>[2x]GSGGSGKVVKFSYMWTINNFSFCREEMGEVIKSSTFSSGANDKLKWCLRVNPKGLDEESKDYLSLYLLLVSCPKSEVRAK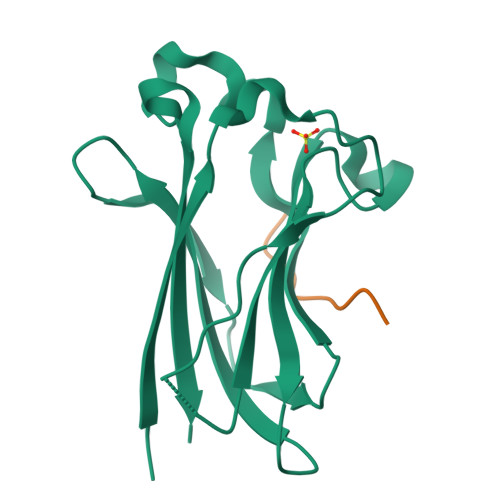FKFSILNAKGEETKAMESQRAYRFVQGKDWGFKKFIRRGFLLDEANGLLPDDKLTLFCEVSVVQD;>[2x]ENLACDEVTSTTSSST> HHHHHHLVPRGSVHHIKRRDIVLKWELGEGAFGKVFLAECHNLLPEQDKMLVAVKALKEASESARQDFQREAELLTMLQHQHIVRFFGVCTEGRPLLMVFEYMRHGDLNRFLRSHGPDAKLLAGGEDVAPGPLGLGQLLAVASQVAAGMVYLAGLHFVHRDLATRNCLVG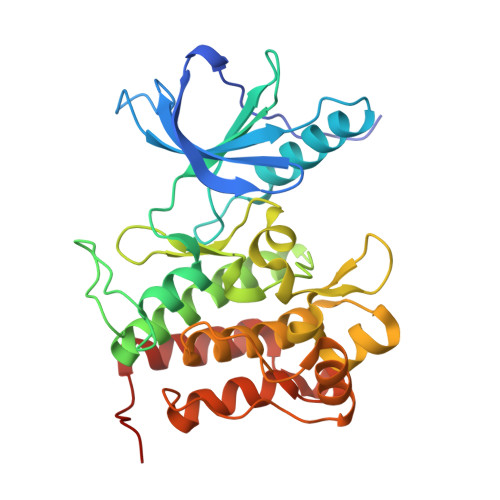QGLVVKIGDFGMSRDIYSTDYYRVGGRTMLPIRWMPPESILYRKFTTESDVWSFGVVLWEIFTYGKQPWYQLSNTEAIDCITQGRELERPRACPPEVYAIMRGCWQREPQQRHSIKDVHARLQALAQAPPVYLDVLG> GPMSKKLSVQEIILTLQKFWSDQGCMLMQSYDTEKGAGTMSPYTFLRAIGPEPWNAAYVEPSRRPADGRYGENPNRLYQHHQFQVVMKPSPENVQDLYLQSLEKLGINPLEHDIRFVE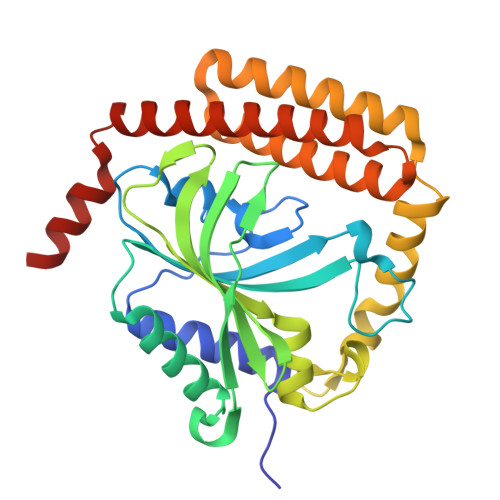DNWENPSMGCAGVGWEVWLDGMEISQFTYFQQVGGLEVDPVTSEITYGLERLSSYIQDVNSVFDLEWGDGVKYGDIFLEPEFENSKYAFEDSNEELLLMLFDEYEKEAKRQIKNGLVHPAYDYCLKCSHTFNLMDARGMVSVTERAGYLDRIRNMAKSIAKEFVAQREKRGFPLLKHAQEETK> MSAAMLLAPGDVIKRSSEELKQRQIQINLIDWTEGESEKESKAEAKEGDKAEELKDGEGTQSESSQKKESSKETKDADVDRRIHTAVGSGSSAKGPGERANENVDRGDGKVGGGGGDADAGVGATGANGGRWVVLTEEIARAIESKYGTKIDVYRDEVPAQIIEVERSLQKELGISREGVAEQTERLRDLRRKEKSGAHAKAAERGRRKQGKKPHGDAQREGTEEEKTSEEPASVGITIEGVMSQKKLLSMIGGVERKMAPIGARESAVMLVSNS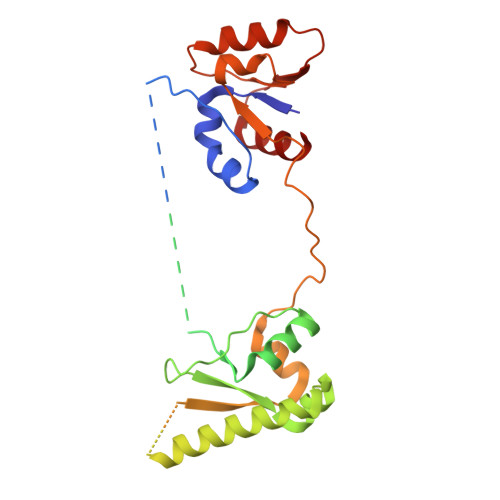IKDVVRATAYFTAPTGDPHWKEVAREASKKKNILAYTSTGGDVKTEFLHLIDHL>[4x]MSKLSVFFIFLFCSIATAAESLPDLKIEKLDEGVYVHTSFEEVNGWGVVPKHGLVVLVNAEAYLIDTPFTAKDTEKLVTWFVERGYKIKGSISSHFHSDSTGGIEWLNSRSIPTYASELTNELLKKDGKVQATNSFSGVNYWLVKNKIEVFYPGPGHTPDNVVVWLPERKILFGGCFIKPYGLGNLGDANIEAWPKSAKLLKSKYGKAKLVVPSHSEVGDASLLKLTLEQAVKGLNESKKPSKPSN

IMP-type metallo-β-lactamases confer resistance to carbapenems and a broad spectrum of β-lactam antibiotics. IMP-6 and IMP-1 differ by only a point mutation: Ser262 in IMP-1 and Gly262 in IMP-6. The overall structures of IMP-6 and IMP-1 are similar.

Here, we report the crystal structures of IMP-6 and IMP-1 with the same space group and similar cell constants at resolutions of 1.70 and 1.94 Å, respectively. The kcat/Km values of IMP-1 for imipenem and meropenem are nearly identical; however, for IMP-6, the kcat/Km for meropenem is 7-fold that for imipenem. However, the loop region (residues 60–66), which participates in substrate binding, is more flexible in IMP-6 than in IMP-1. This difference in flexibility determines the substrate specificity of IMP-type metallo-β-lactamases for imipenem and meropenem. The amino acid at position 262 alters the mobility of His263; this affects the flexibility of the loop via a hydrogen bond with Pro68, which plays the role of a hinge in IMP-type metallo-β-lactamases.We present the structural and functional characterisation of a subtilase autotransporter, Ssp, from the opportunistic pathogen Serratia marcescens. Autotransporters (ATs) are the largest family of secreted proteins in Gram-negative bacteria with many having important roles in bacterial infection and disease, including adhering to and invading host cells, biofilm formation along with being potent cytotoxins and immunomodulators. Subtilase ATs comprise one of the two AT families which possess protease activity, with the other being the (chymo)trypsin-like protease ATs which include SPATEs (serine protease autotransporters of Enterobactericeae). We further reveal that the activity of the subtilase AT is required for entry into epithelial cells as well as causing cellular toxicity.

A number of SeMet datasets were merged, which were used along with the Ssp model to solve the structure using single isomorphous replacement with anomalous scattering (SIRAS) and molecular replacement with single wavelength anomalous diffraction (MRSAD). One molecule of Ssp is present in the asymmetric unit, where the resulting structure was refined against a higher resolution native (2.0 Å) dataset with a final and Rfactor/Rfree of 16.3/20.1 (crystallographic statistics in Table 1). The subtilase domain of Ssp is positioned directly on top of the β-helical domain, essentially capping the β-helical scaffold. The core architecture of the protease domain of Ssp is typical of the subtilisin-like folds observed in other subtilase enzymes. It is comprised of a globular α/β fold centrally featuring a twisted seven-stranded parallel β-sheet adjacent to two central α-helices and encompassing the active site residues D76, H112 and S341. A disulfide bond (Cys288 to Cys295) connects the last β-strand of the β-sheet to its preceding loop. In comparison to the subtilisin BPN’, the catalytic triad sits at the bottom of a deep cleft formed by two protruding β-hairpins (E1 and E3) on one side and an extended loop (E2) on the other which are absent from subtilisin BPN’. Ssp harbours a deletion, equivalent to residues 98–109 of subtilisin BPN’, adjacent to the subtilisin BPN’ S4 subsite. This results in a truncated α-helix and makes the binding cleft wider, which conceivably allows for a more extensive substrate binding interface. Interestingly, the Ssp β-helix is the shortest seen to date for an AT, comprising of seven right-handed triangular turns (~40 Å in length), with the last three β-strand rungs resembling an autochaperone domain, which previous studies have shown are involved in AT passenger folding. The structural characterisation of Ssp revealed the presence of three calcium binding sites, two in the subtilase domain and one in the β-helical stalk domain.

> AYQDPGRLGAPDSWKTAEFNRQWGLEAISAEFAYARGYTGKGITIGVIDNAILSHSEFSGKLTRLDNGSYNFSYDKQDNMSFGDHGTHVAGIAAAKRDGAGMHGVAFDADIIGTKLNDYGNRNGREELIQSAARVINNSWGIAPDIRRDAKGDIIWLPNGRPDYVAFVKSEVIAEMMRSKSSVEWGSEQPVPTGGHSAMSTLLRAARHGKLIVFSAGNYNNYNIPEAQKSLPYAFPDVLNNYLIVTNLSDENQLSVSSTSCGQTASYCVSAPGSDIYSTVGRLESNTGGAVNREAYNKGELSLNPGYGNKSGTSMAAPHVTGVAAVLMQRFPYMSADQISAVIKTTATDLGVAGIDNLFGWGRVNLRDAINGPKMFITKEDIPQEYYVPGSYSEKQFVVNIPGLGNIVEPGTPVERRCTSSECSFDSWSNDISGHGGLTKTGAGTLALLGNNTYRGDTWVKQGVLAIDGSVASNVYIENSGTLSGEGTVGAFRAARSGSVAPGNGIGTLHVLHDAIFDRGSQYNVEVADNGRSDKIAARRAFLNGGSVNVSLERSQNLLSQNEAQSLLGNKYTILTTTDGVTGRFENANPSYPFVKVALDYRGNDVGLGITRTDASFD> MEEDKLALGREIFLERSEPQCALCHTLADAEAVGEVGPNLDELKPDAERVNTAV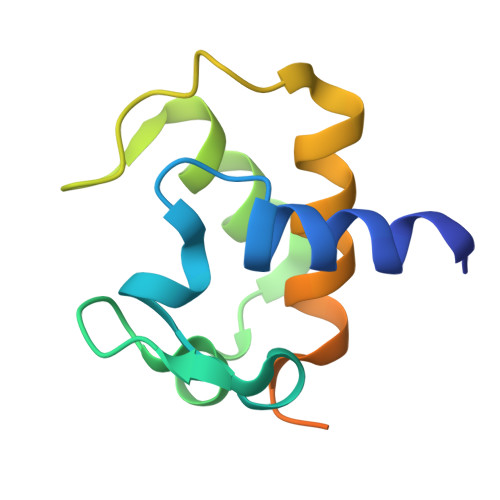TNGIGPMPANEILTDEEIEAVALYVSTVAGKAKNSSSVDKLAAALEHHHHHH4-{4-[6-(2-methoxyethoxy)quinolin-2-yl]-1H-1,2,3-triazol-1-yl}phenol | C20 H18 N4 O3 | 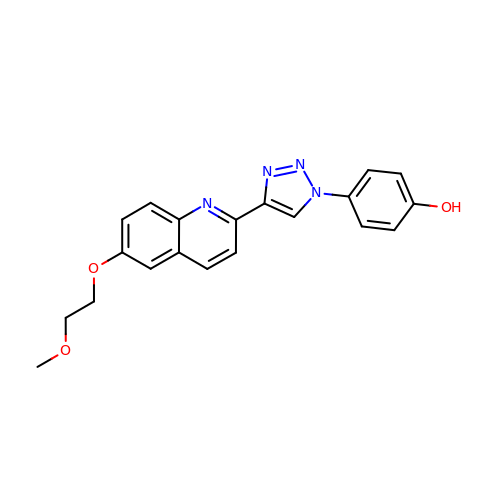RDMXBXKUWXFIGH-UHFFFAOYSA-N> MSADAQSFLNRVCGVSAARLTPCGTGTSTDVVYRAFDIYNDKVAGFAKFLKTNCCRFQEKDEDDNLIDSYFVVKRHTFSNYQHEETIYNLLKDCPAVAKHDFFKFRIDGDMVPHISRQRLTKYTMADLVYALRHFDEGNCDTLKEILVTYNCCDDDYFNKKDWYDFVENPDILRVYANLGERVRQALLKTVQFCDAMRNAGIVGVLTLDNQDLNGNWYDFGDFIQTTPGSGVPVVDSYYSLLMPILTLTRALTAESHVDTDLTKPYIKWDLLKYDFTEERLKLFDRYFKYWDQTYHPNCVNCLDDRCILHCANFNVLFSTVFPPTSFGPLVRKIFVDGVPFVVSTGYHFRELGVVHNQDVNLHSSRLSFKELLVYAADPAMHAASGNLLLDKRTTCFSVAALTNNVAFQTVKPGNFNKDFYDFAVSKGFFKEGSSVELKHFFFAQDGNAAISDYDYYRYNLPTMCDIRQLLFVVEVVDKYFDCYDGGCINANQVIVNNLDKSAGFPFNKWGKARLYYDSMSYEDQDALFAYTKRNVIPTITQMNLKYAISAKNRARTVAGVSICSTMTNRQFHQKLLKSIAATRGATVVIGTSKFYGGWHNMLKTVYSDVENPHLMGWDYPKCDRAMPNMLRIMASLVLARKHTTCCSLSHRFYRLANECAQVLSEMVMCGGSLYVKPGG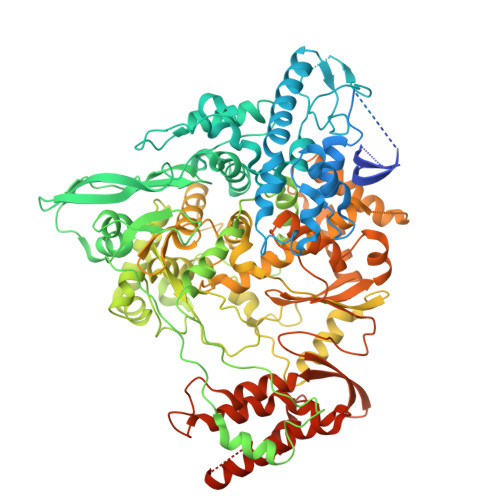TSSGDATTAYANSVFNICQAVTANVNALLSTDGNKIADKYVRNLQHRLYECLYRNRDVDTDFVNEFYAYLRKHFSMMILSDDAVVCFNSTYASQGLVASIKNFKSVLYYQNNVFMSEAKCWTETDLTKGPHEFCSQHTMLVKQGDDYVYLPYPDPSRILGAGCFVDDIVKTDGTLMIERFVSLAIDAYPLTKHPNQEYADVFHLYLQYIRKLHDELTGHMLDMYSVMLTNDNTSRYWEPEFYEAMYTPHTVLQLEHHHHHH>[4x]KEWQENKSWNAHFTEHKSQGVVVLWNENKQQGFTNNLKRANQAFLPASTFKIPNSLIALDLGVVKDEHQVFKWDGQTRDIATWNRDHNL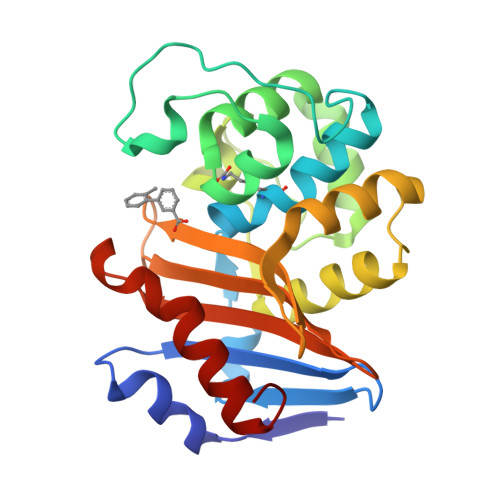ITAMKYSVVPVYQEFARQIGEARMSKMLHAFDYGNEDISGNVDSFWLDGGIRISATEQISFLRKLYHNKLHVSERSQRIVKQAMLTEANGDYIIRAKTGYSTRIEPKIGWWVGWVELDDNVWFFAMNMDMPTSDGLGLRQAITKEVLKQEKIIP2-[[3-(7-bromanyl-1,2,4,5-tetrahydro-3-benzazepin-3-yl)-1,2,4-oxadiazol-5-yl]methyl]-3,4-dihydro-1~{H}-isoquinoline-7-carboxylic acid | C23 H23 Br N4 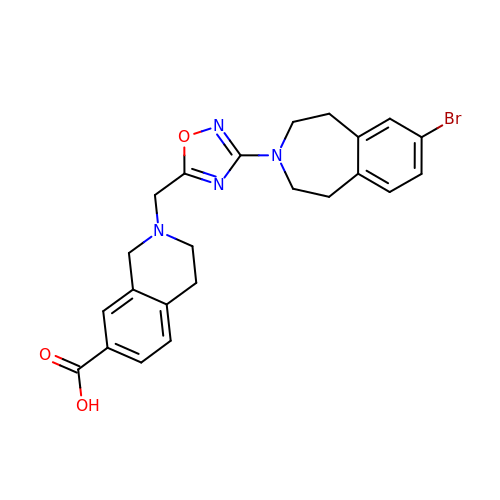O3 | LMIHZOOKIJYEAW-UHFFFAOYSA-N> MADHNKKDVGSWASPNEHLMFFDFSSWLLVDFGKRWERWVSFKKSFLTTTRSPY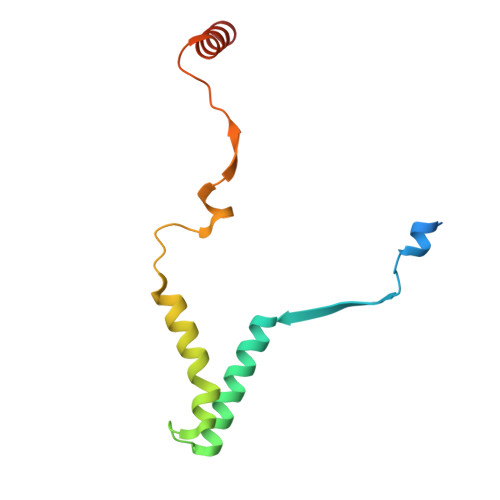WSPQFFLLTFFQLRNSNVKLCENWNWAPKGDDFNLLHNSAAEPFGRDLKAHLEREAGAKHHH> VNPCCYYPCQHQGICVRFGLDRYQCDCTRTGYSGPNCTIPEIWTWLRTTLRPSPSFIHFLLTHGRWLWDFVNATFIRDTLMRLVLTVRSNLIPSPPTYNIAHDYISWESFSNVSYYTRILPSVPRDCPTPMGTKGKKQLPDAEFLSRRFLLRRKFIPDPQGTNLMFAFFAQHFTHQFFKTSGKMGPGFTKALGHGVDLGHIYGDNLERQYQLRLFKDGKLKYQMLNGEVYPPSVEEAPVLMHYPRGIPPQSQMAVGQEVFGLLPGLMLYATIWLREHNRVCDLLKAEHPTWGDEQLFQTARLILIGETIKIVIEEYVQQLSGYFLQLKFDPELLFGAQFQYRNRIAMEFNQLYHWHPLMPDSFRVGPQDYSYEQFLFNTSMLVDYGVEALVDAFSRQPAGRIGGGRNIDHHILHVAVDVIKESRVLRLQPFNEYRKRFGMK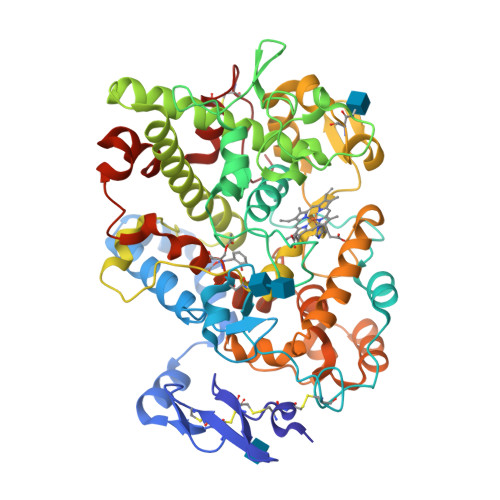PYTSFQELTGEKEMAAELEELYGDIDALEFYPGLLLEKCHPNSIFGESMIEMGAPFSLKGLLGNPICSPEYWKASTFGGEVGFNLVKTATLKKLVCLNTKTCPYVSFHVP4-hydroxy-8-nitroquinoline-3-carboxylic 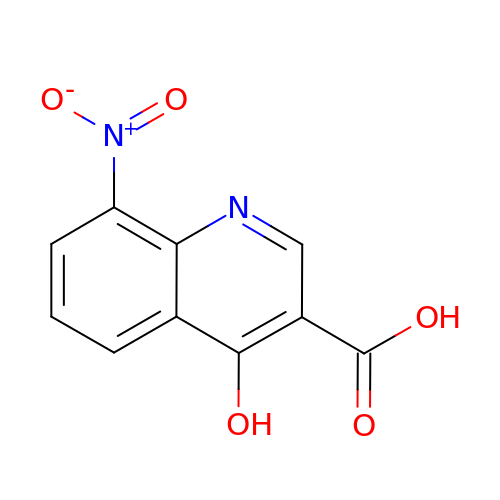acid | C10 H6 N2 O5 | BMIZBCVEHSUUNO-UHFFFAOYSA-N>ASTKAQPTEVSSILEERIKGVSDEANLNETGRVLAVGDGIARVFGLNNIQAEELVEFSSGVKGMALNLEPGQVGIVLFGSDRLVKEGELVKRTGNIVDVPVGPGLLGRVVDALGNPIDGKGPIDAAGRSRAQVKAPGILPRRSVHEPVQTGLKAVDALVPIGRGQRELIIGDRQTGKTAVALDTILNQKRWNNGSDESKKLYCVYVAVGQKRSTVAQLVQTLEQHDAMKYSIIVAATASEAAPLQYLAPFTAASIGEWFRDNGKHALIVYDDLSKQAVAYRQLSLLLRRPPGREAYPGDVFYLHSRLLERAAKLSEKEGSGSLTALPVIETQGGDVSAYIPTNVISITDGQIFLEAELFYKGIRPAINVGLSVSRVGSAAQVKALKQVAGSLKLFLAQYREVAAFAQFGSDLDASTKQTLVRGERLTQLLKQNQYSPLATEEQVPLIYAGVNGHLDGIELSRIGEFESSFLSYLKSNHNELLTEIREKGELSKELLASLKSATESFVATF[6x];>[6x]ASAAQSTPITGKVTAVIGAIVDVHFEQSELPAILNALEIKTPQGKLVLEVAQHLGENTVRTIAMDGTEGLVRGEKVLDTGGPISVPVGRETLGRIINVIGEPIDERGPIKSKLRKPIHADPPSFAEQSTSAEILETGIKVVDLLAPYARGGKIGLFGGAGVGKTVFIQELINNIAKAHGGFSVFTGVGERTREGNDLYREMKETGVINLEGESKVALVFGQMNEPPGARARVALTGLTIAEYFRDEEGQDVLLFIDNIFRFTQAGSEVSALLGRIPSAVGYQPTLATDMGLLQERITTTKKGSVTSVQAVYVPADDLTDPAPATTFAHLDATTVLSRGISELGIYPAVDPLDSKSRLLDAAVVGQEHYDVASKVQETLQTYKSLQDIIAILGMDELSEQDKLTVERARKIQRFLSQPFAVAEVFTGIPGKLVRLKDTVASFKAVLEGKYDNIPEHAFYMVGGIEDVVAKAEKLAAEAN;>ATLKEVEMRLKSIKNIEKITKTMKIVASTRLSKAEKAKISAKKMDEAEQLFYKNAETKNLDVEATETGAPKELIVAITSDKGLCGSIHSQLAKAVRRHLNDQPNADIVTIGDKIKMQLLRTHPNNIKLSINGIGKDAPTFQESALIADKLLSVMKAGTYPKISIFYNDPVSSLSFEPSEKPIFNAKTIEQSPSFGKFEIDTDANVPRDLFEYTLANQMLTAMAQGYAAEISARRNAMDNASKNAGDMINRYSILYNRTRQAVITNELVDIITGASSLG[2x];>AEAAAASSGLKLQFALPHETLYSGSEVTQVNLPAKSGRIGVLANHVPTVEQLLPGVVEVMEGSNSKKFFISGGFATVQPDSQLCVTAIEAFPLESFSQENIKNLLAEAKKNVSSSDAREAAEAAIQVEVLENLQSVLK[2x];>SAWRKAGISYAAY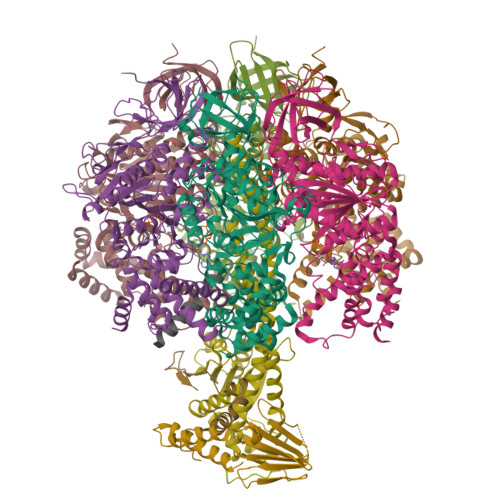LNVAAQAIRSSLKTELQTASVLNRSQTDAFYTQYKNGTAASEPTPITK[2x];>SEGSTGTPRGSGSEDSFVKRARATEDFFVRQREKEQLRHLKEQLEKQRKKIDSLENKIDSMTK[2x]> VHFHPFGNVNFYEMDWSLKGDLWAHAPVIAKEGSRWYVFHTGSGIQIKTSEDGVHWENMGWVFPSLPDWYKQYVPEKDEDHLWAPDICFYNGIYYLYYSVSTFGKNTSVI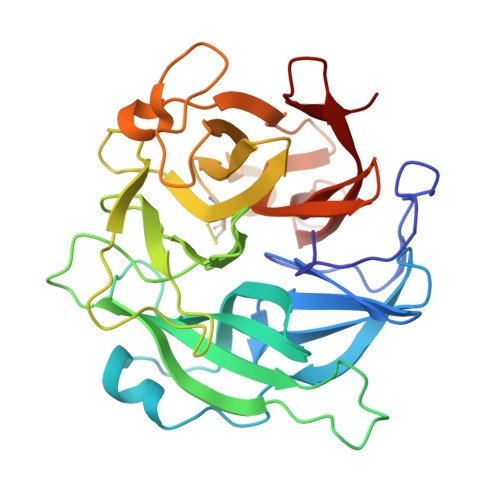GLATNQTLDPRDPDYEWKDMGPVIHSTASDNYNAIDPNVVFDQEGQPWLSFGSFWSGIQLIQLDTETMKPAAQAELLTIASRGEEPNAIEAPFIVCRNGYYYLFVSFDFCCRGIESTYKIAVGRSKDITGPYVDKNGVSMMQGGGTILDEGNDRWIGPGHCAVYFSGVSAILVNHAYDALKNGEPTLQIRPLYWDDEGWPYLSV> GFRASRSHSRREEHSGRNGLHHPSPDHFWPRFPDALRPFVPWDQLENEDSSVHISPRQKRDAN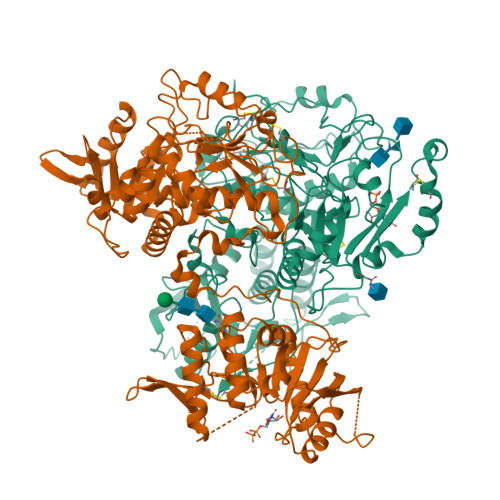SSIYKGKKCRMESCFDFTLCKKNGFKVYVYPQQKGEKIAESYQNILAAIEGSRFYTSDPSQACLFVLSLDTLDRDQLSPQYVHNLRSKVQSLHLWNNGRNHLIFNLYSGTWPDYTEDVGFDIGQAMLAKASISTENFRPNFDVSIPLFSKDHPRTGGERGFLKFNTIPPLRKYMLVFKGKRYLTGIGSDTRNALYHVHNGEDVVLLTTCKHGKDWQKHKDSRCDRDNTEYEKYDYREMLHNATFCLVPRGRRLGSFRFLEALQAACVPVMLSNGWELPFSEVINWNQAAVIGDERLLLQIPSTIRSIHQDKILALRQQTQFLWEAYFSSVEKIVLTTLEIIQDRIFKHISRNSLIWNKHPGGLFVLPQYSSYLGDFPYYYANLGLKPPSKFTAVIHAVTPLVSQSQPVLKLLVAAAKSQYCAQIIVLWNCDKPLPAKHRWPATAVPVVVIEGESKVMSSRFLPYDNIITDAVLSLDEDTVLSTTEVDFAFTVWQSFPERIVGYPARSHFWDNSKERWGYTSKWTNDYSMVLTGAAIYHKYYHYLYSHYLPASLKNMVDQLANCEDILMNFLVSAVTKLPPIKVTQKKQYKETMMGQTSRASRWADPDHFAQRQSCMNTFASWFGYMPLIHSQMRLDPVLFKDQVSILRKKYRDIERL;> WPHSIESSNDWNVEKRSIRDVPVVRLPADSPIPERGDLSCRMHTCFDVYRCGFNPKNKIKVYIYALKKYVDDFGVSVSNTISREYNELLMAISDSDYYTDDINRACLFVPSIDVLNQNTLRIKETAQAMAQLSRWDRGTNHLLFNMLPGGPPDYNTALDVPRDRALLAGGGFSTWTYRQGYDVSIPVYSPLSAEVDLPEKGPGPRQYFLLSSQVGLHPEYREDLEALQVKHGESVLVLDKCTNLSEGVLSVRKRCHKHQVFDYPQVLQEATFCVVLRGARLGQAVLSDVLQAGCVPVVIADSYILPFSEVLDWKRASVVVPEEKMSDVYSILQSIPQRQIEEMQRQARWFWEAYFQSIKAIALATLQIINDRIYPYAAISYEEWNDPPAVKWGSVSNPLFLPLIPPQSQGFTAIVLTYDRVESLFRVITEVSKVPSLSKLLVVWNNQNKNPPEDSLWPKIRVPLKVVRTAENKLSNRFFPYDEIETEAVLAIDDDIIMLTSDELQFGYEVWREFPDRLVGYPGRLHLWDHEMNKWKYESEWTNEVSMVLTGAAFYHKYFNYLYTYKMPGDIKNWVDAHMNCEDIAMNFLVANVTGKAVIKVTPRKKFKCPECTAIDGLSLDQTHMVERSECINKFASVFGTMPLKVVEHRADPVLYKDDFPEKLKSFPNIGSL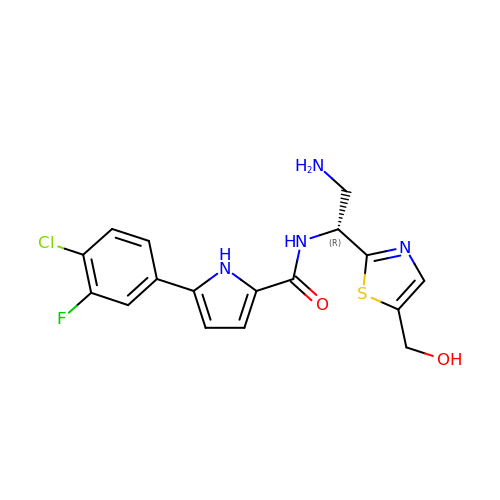~{N}-[(1~{R})-2-azanyl-1-[5-(hydroxymethyl)-1,3-thiazol-2-yl]ethyl]-5-(4-chloranyl-3-fluoranyl-phenyl)-1~{H}-pyrrole-2-carboxamide | C17 H16 Cl F N4 O2 S | BCGYPAUBMXRDJQ-OAHLLOKOSA-N(2S)-2-methylbutanedioic acid | C5 H8 O4 | 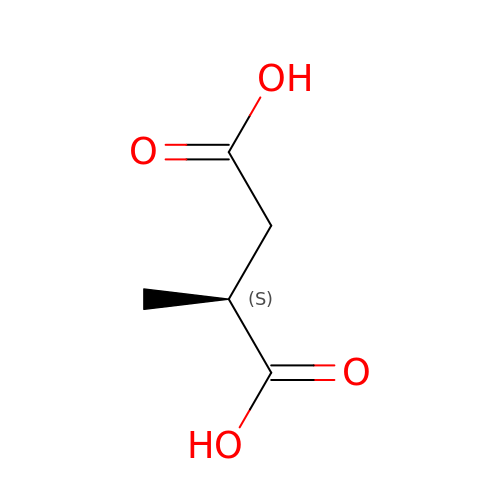WXUAQHNMJWJLTG-VKHMYHEASA-N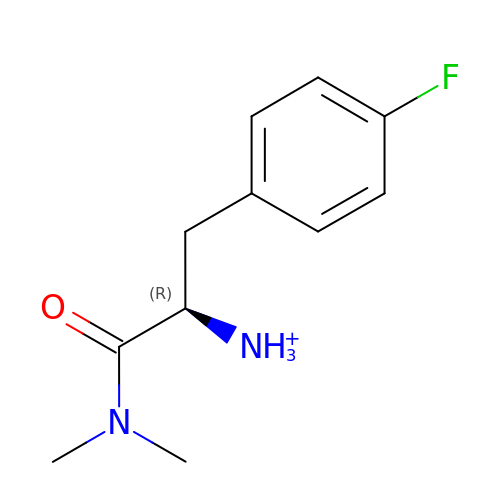[(2~{R})-1-(dimethylamino)-3-(4-fluorophenyl)-1-oxidanylidene-propan-2-yl]azanium | C11 H16 F N2 O | SLKQPFCNEFCUMC-SNVBAGLBSA-O> SRAPDQDEIQRLPGLAKQPSFRQYSGYLKGSGSKHLHYWFVESQKDPENSPVVLWLNGGPGCSSLDGLLTEHGPFLVQPDGVTLEYNPYSWNLIANVLYLESPAGVGFSYSDDKFYATNDTEVAQSNFEALQDFFRLFPEYKNNKLFLTGESYAGIYIPTLAVLVMQDPSMNLQGLAVGNGLSSYEQNDNSLVYFAYYHGLLGNRLWSSLQTHCCSQNKCNFYDNKDLECVTNLQEVARIVGNSGLNIYNLYAPCAGGVPSHFRYEKDTVVVQDLGNIFTRLPLKRMWHQALLRSGD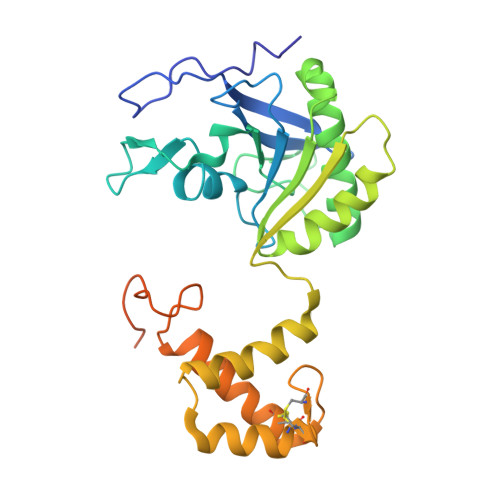KVR3-{[(1R)-1-phenylethyl]amino}-4-(pyridin-4-ylamino)cyclobut-3-ene-1,2-dione | C17 H15 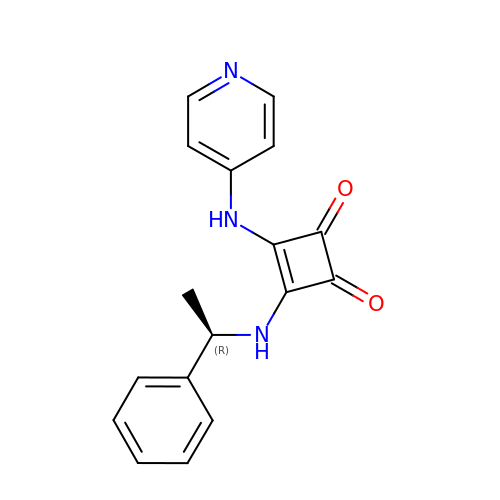N3 O2 | MCBPNFWHHNJTGN-LLVKDONJSA-N>GSKETAFVEVVLFESSPSGDYTTHTTGLTGRFSRAGAMLSAEGEIVQMHPLGLCNNNDEEDLYEYGWVGVVKLEQPELDPKPCLTVLGKAKRAVQRGATAVIFDVSENPEAIDQLNQGSEDPLKRPVVYVKGADAIKLMNIVNKQKVARARIQHLAAAHHHHHH[2x]

Zinc RING finger 3 (ZNRF3) and its homolog RING finger 43 (RNF43) are trans-membrane E3 ubiquitin ligases that negatively regulate Wnt signaling. ZNRF3 and RNF43 contain an extracellular N-terminal protease-associated (PA) domain, a single pass trans-membrane helix and an intracellular C-terminal RING domain with E3 ligase activity. Interaction of ZNRF3 or RNF43 with complexes of frizzled receptors (FZD) and low-density lipoprotein receptor-related protein (LRP) 5/6 leads to Frizzled ubiquitination and endocytosis of the heterodimeric receptors, thereby reducing the capacity of Wnt-driven signal transduction. RNF43 and its homolog ZNRF3 have been identified as E3 ligases that ubiquitinate Frizzled receptors for degradation, whereas RSPO1 captures ZNRF3 for removal from membrane, thereby increasing Frizzled expression on the cell surface.

Purified protein was crystallized and crystals exhibited space group P21 with cell dimensions a = 35.7 Å, b = 73.5 Å and c = 58.6 Å and β = 97.5°, contained two molecules per asymmetric unit and diffracted to 1.5 Å resolution. The ZNRF3 ectodomain adopts a typical PA-fold, previously found in e.g. subtilases, transferrin receptors and vacuolar sorting receptors. The central core of the molecule is formed by a parallel β-sheet, consisting of strands β3-β4-β5-β6 surrounded by three α-helices and two short 310-helices. A disulphide bond Cys107-Cys136, which is present in both ZNRF3 and RNF43 connects the loop regions containing the first and second 310-helices. The N-terminal and C-terminal residues of the ectodomain form an anti-parallel β-sheet, β2-β1-β7, that packs against helix α3. In ZNRF3, strands β1 and β2 form an extended β-hairpin ‘flap’, while RNF43 is three residues shorter and displays a flexible loop in this region. In the crystal structure of ZNRF3, we observe two molecules in the asymmetric unit. The two molecules pack together making an extensive interface burying over ~1,000 Å2 surface area. In addition, we observe stacking of guanidinium groups of Arg178-Arg204’. Both C-termini of the dimer point to the same direction, making such arrangement plausible on the membrane. However, at present it is not clear if such arrangement is physiologically relevant.>[2x]RPLAFSDAGPHVHYG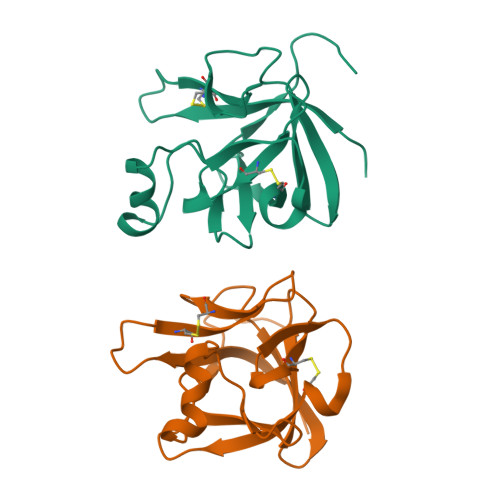WGDPIRLRHLYTSGPHGLSSCFLRIRADGVVDCARGQSAHSLLEIKAVALRTVAIKGVHSVRYLCMGADGKMQGLLQYSEEDCAFEEEIRPDGYNVYRSEKHRLPVSLSSAKQRQLYKNRGFLPLSHFLPMLPMVPEEPEDLRGHLESDMFSSPLETDSMDPFGLVTGLEAVRSPSFEK>[2x]HMK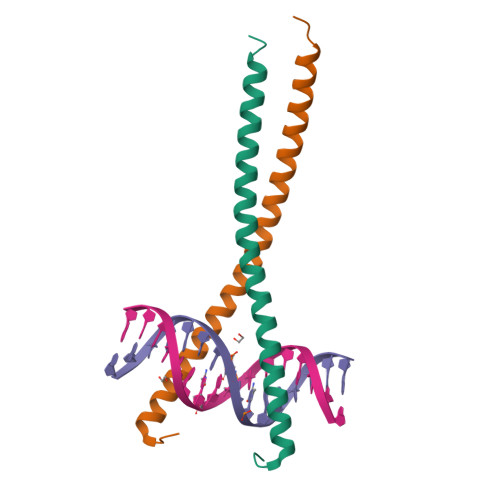HSDEYKIRRERNNIAVRKSRDKAKMRNLETQHKVLELTAENERLQKKVEQLSRELSTLRNLFKQLPEPLLASSGH> MAAHLSYGRVNLNVLREAVRRELREFLDKCAGSKAIVWDEYLTGPFGLIAQYSLLKEHEVEKMFTLKGNRLPAADVKNIIFFVRPRLELMDIIAENVLSEDRRGPTRDFHILFVPRRSLL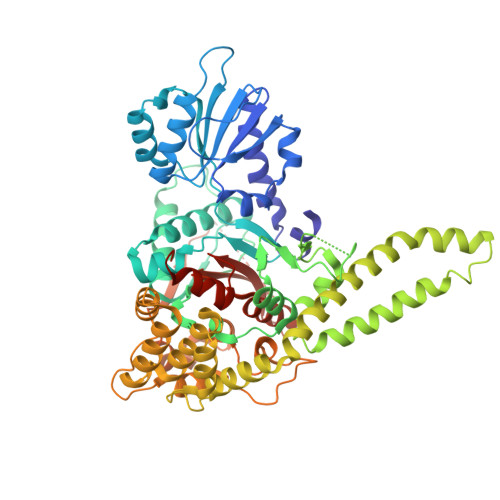CEQRLKDLGVLGSFIHREEYSLDLIPFDGDLLSMESEGAFKECYLEGDQTSLYHAAKGLMTLQALYGTIPQIFGKGECARQVANMMIRMKREFTGSQNSIFPVFDNLLLLDRNVDLLTPLATQLTYEGLIDEIYGIQNSYVKLPPEKFAPKKQGDGGKDLPTEAKKLQLNSAEELYAEIRDKNFNAVGSVLSKKAKIISAAFEERHNAKTVGEIKQFVSQLPHMQAARGSLANHTSIAELIKDVTTSEDFFDKLTVEQEFMSGIDTDKVNNYIEDCIAQKHSLIKVLRLVCLQSVCNSGLKQKVLDYYKREILQTYGYEHILTLHNLEKAGLLKPQTGGRNNYPTIRKTLRLWMDDVNEQNPTDISYVYSGYAPLSVRLAQLLSRPGWRSIEEVLRILPGPHFEERQPLPTGLQKKRQPGENRVTLIFFLGGVTFAEIAALRFLSQLEDGGTEYVIATTKLMNGTSWIEALMEKPFHHHHHHHHHH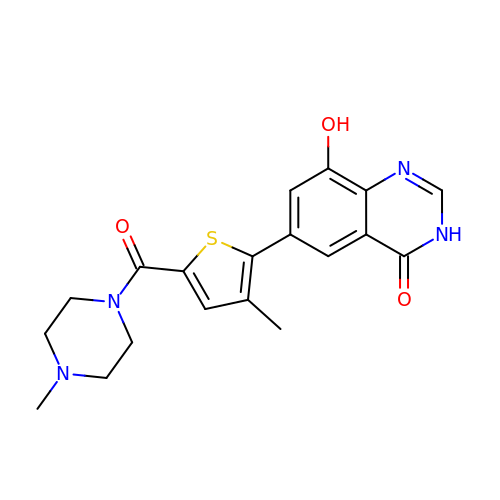6-[3-methyl-5-(4-methylpiperazin-1-yl)carbonyl-thiophen-2-yl]-8-oxidanyl-3~{H}-quinazolin-4-one | C19 H20 N4 O3 S | DNJWFDOPNCCIRY-UHFFFAOYSA-N> MPKLVTWMNNQRVGELTKLANGAHTFKYAPEWLASRYARPLSLSLPLQRGNITSDAVFNFFDNLLPDSPIVRDRIVKRYHAKSRQPFDLLSEIGRDSVGAVTLIPEDETVTHP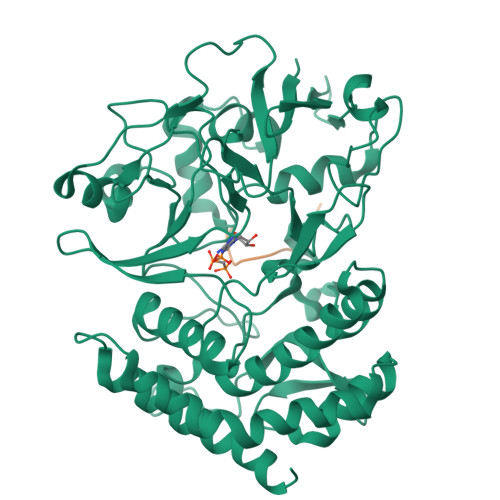IMAWEKLTEARLEEVLTAYKADIPLGMIREENDFRISVAGAQEKTALLRIGNDWCIPKGITPTTHIIKLPIGEIRQPNATLDLSQSVDNEYYCLLLAKELGLNVPDAEIIKAGNVRALAVERFDRRWNAERTVLLRLPQEDMCQTFGLPSSVKYESDGGPGIARIMAFLMGSSEALKDRYDFMKFQVFQWLIGATQGHAKNFSVFIQAGGSYRLTPFYDIISAFPVLGGTGIHISDLKLAMGLNASKGKKTAIDKIYPRHFLATAKVLRFPEVQMHEILSDFARMIPAALDNVKTSLPTDFPENVVTAVESNVLRLHGRLSREY> MDLLKKEYTGITYISGPLLFVENAKDLAYGAIVDIKDGTGRVRGGQVIEVSEEYAVIQVFEETTGLDLATTSVSLVEDVARLGVSKEMLGRRFNGIGKPIDGLPPITPEKRLPITGLPLNPVARRKPEQFIQTGISTIDVMNTL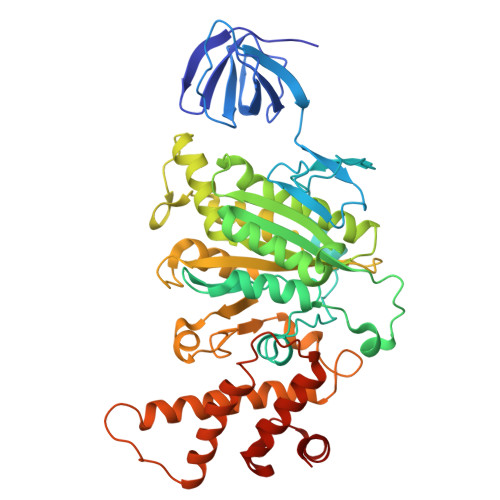VRGQKLPIFSGSGLPANEIAAQIARQATVRPDLSGEGEKEEPFAVVFAAMGITQRELSYFIQEFERTGALSRSVLFLNKADDPTIERILTPRMALTVAEYLAFEHDYHVLVILTDMTNYSEALREIGAAREEIPGRRGYPGYMYTDLATIYERAGVVEGKKGSVTQIPILSMPDDDRTHPIPDLTGYITEGQIQLSRELHRKGIYPPIDPLPSLSRLMNNGVGKGKTREDHKQVSDQLYSAYANGVDIRKLVAIIGEDALTENDRRYLQFADAFERFFINQGQQNRSIEESLQIAWALLSMLPQGELKRISKDHIGKYYG>[2x]MTEGSVARQPDLSTCDDEPIHIPGAIQPHGLLLALAADMTIVAGSDNLPELTGLAIGALIGRSAADVFDSETHNRLTIALAEPGAAVGAPIAVGFTMPDGERAFNGSWHRHDQLVFLELEPPQRDVR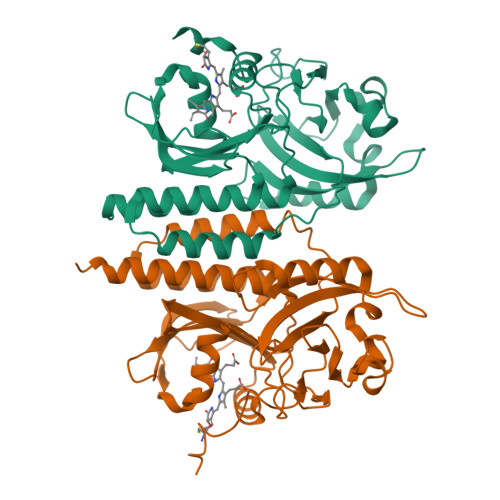YPQAFFRSVRSAIRRLQAAETLESACAAAAQEVREITGFDRVMIYRFASDFSGEVIAEDRCAEVESYLGLHFPASDIPAQARRLYTINPVRIIPDINYRPVPVTPDLNPRTGRPIDLSFAILRSVSPVHLEYMRNIGMHGTMSISILRGERLWGLIACHHRKPNYVDLEVRQACELVAQVLAWQIGVMEEQALEHHHHHH>GPGGSGGMKPQIRNMVEPMDPRTFVSNFNNRPILSGLDTVWLCCEVKTKDPSGPPLDAKIFQGKVYPKAKYHPEMRFLRWFHKWRQLHHDQEYKVTWYVSWSPCTRCANSVATFLAKDPKVTLTIFVARLYYFWDPDYQQALRILAEAGATMKIMNYNEFQDCWNKFVDGRGKPFKPWNNLPKHYTLLQATLGELLRHLMDPGTFTSNFNNKPWVSGQHETYLCYKVERLHNDTWVPLNQHRGFLRNQAPNIHGFPKGRHAQLCFLD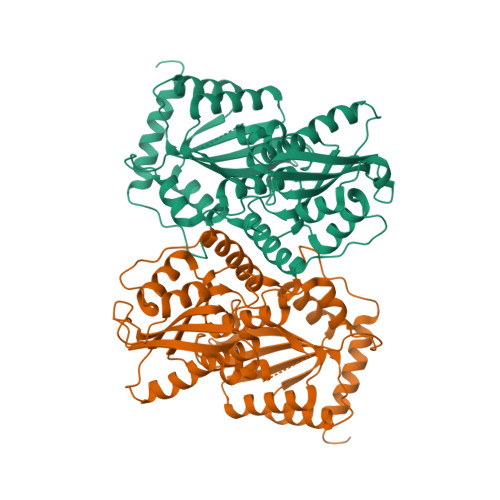LIPFWKLDGQQYRVTCFTSWSPCFSCAQEMAKFISNNEHVSLCIFAARIYDDQGRYQEGLRTLHRDGAKIAMMNYSEFEYCWDTFVDRQGRPFQPWDGLDEHSQALSGRLRAILQNQGN[2x]> MTTNPVDLWSAPSSQARLEKEYFDQHFGPFFRTEQLIIRAPLTDKHIYQPYPSGADVPFGPPLDIQILHQVLDLQIAIENITASYDNETVTLQDICLAPLSPYNTNCTILSVLNYFQNSHSVLDHKKGDDFFVYA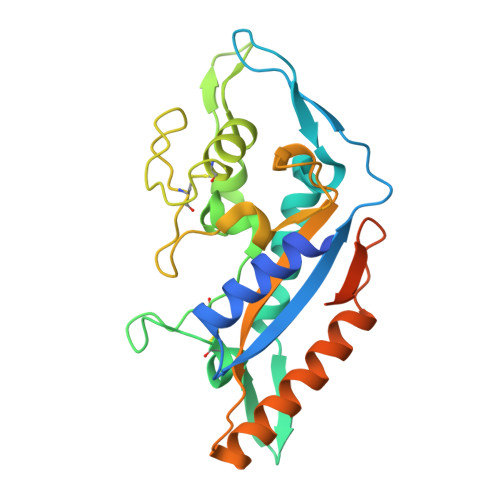DYHTHFLYCVRAPASLNDTSLLHDPCLGTFGGPVFPWLVLGGYDDQNYNNATALVITFPVNNYYNDTEKLQRAQAWEKEFINFVKNYKNPNLTISFTAERSIEDELNRESDSDLEHHHHHH>MAAPSPTTTAAAAAAATTHHRVLLPSARPRAAPSSLRLPLRAQPHAHAHAQRARLAAPVAAAAPAPAASTASPESPASGAVAGKPTVLVAEKLGAAGLALLREFANVDCSYGLSPEDLRAKISLCDALIVRSGTKVGRDVFEASGGRLRVVGRAGVGIDNVDLAAATEHGCLVVNAPTANTVAAAEHGIALLTAMARNIAQADASLKAGKWQRNKYVGVSLVGKTLAILGFGKVGSEVARRAKGLGMHVIAHDPYASADRARAIGVELVSMEEAMTTADFILLHMPLTPATDKMLNDEAFAKMKKGVRIINVARGGVIDEEALVRALDSGVVAQAALDVFTKEPPAADNKLVLHGNVTVTPHLGASTVEAQEGVAIEIAEAVIGALK[2x]

Here, we cloned and functionally characterized the maize (Zea mays) gene Dek20, which encodes phosphoglycerate dehydrogenase1 (PGDH1), the rate-limiting enzyme in the phosphorylated pathway of serine biosynthesis (PPSB). The first step, catalyzed by 3-phosphoglycerate dehydrogenase (PGDH), oxidizes 3-PGA into 3-phosphohydroxypyruvate (3-PHP) and is the rate-limiting reaction. The mature transcript of Dek20 features an 1,881-bp coding sequence, which encodes a protein consisting of 626 amino acids that includes 3 domains: the substrate binding domain (SBD, residues 1-179), the nucleotide-binding domain (NBD, residues 180-367), and the regulatory domain (RBD, residues 388-626). DEK20 and its mammalian homologs are classified as type I PGDH, characterized by 3 major domains: the substrate binding domain, nucleotide-binding domain, and regulatory domains.

Exome sequencing was conducted to uncover variants, which were then filtered against the third-generation Zea mays haplotype map. Among the candidate mutations listed in Supplementary Data Set 1, a C-to-T mutation was identified in the second exon of Zm00001d002051, resulting in a substitution of the 282nd amino acid, from serine (Ser) to leucine (Leu), in dek20. The overall structure of DEK20S282L was quite similar to DEK20WT (R.M.S.D. 0.465 Å). According to the structures, the residue Ser or Leu at 282 was located in NBD but had no direct interaction with NAD + . By contrast, Leu282 had no interaction with His284 in DEK20S282L, resulting in the spatial position of the His284 imidazole group close to NAD+. This change enabled His284 to interact with NAD+ through hydrogen bonds, which may increase the binding affinity and affect the release of NAD+ from DEK20(S282L), and eventually decrease the catalytic activity. The dissociation constant (Kd) of DEK20 was found to be 32.45 μM, while for DEK20(S282L), it is 8.11 μM. These results indicate that the S282L mutation significantly enhances DEK20's binding ability to NAD+. To determine whether this enhancement resulted from the interaction of His284 with NAD+, we mutated His284 to Ala (H284A) and observed that the H284A mutation reversed the increase of NAD+ affinity of DEK20(S282L). Notably, the wild-type DEK20 exhibited superior enzyme activity compared to its mutated variant, DEK20(S282L). Correspondingly, the decreased enzyme activity of DEK20(S282L) was also restored by the H284A mutation.> HLE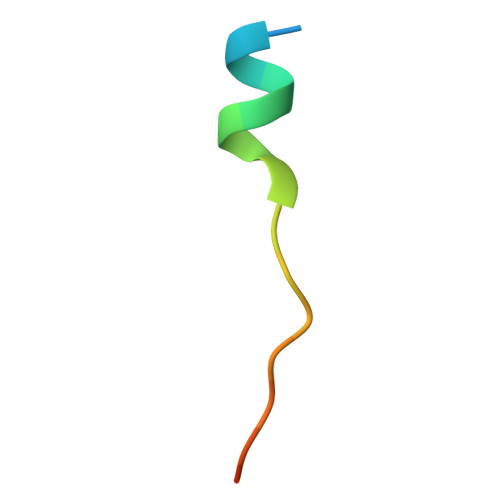VVKLLLEHGADVXAQDK~{N}-[(2~{R})-2-(4-nitrophenyl)-2-oxidanyl-ethyl]-1,3-benzodioxole-5-carboxamide | 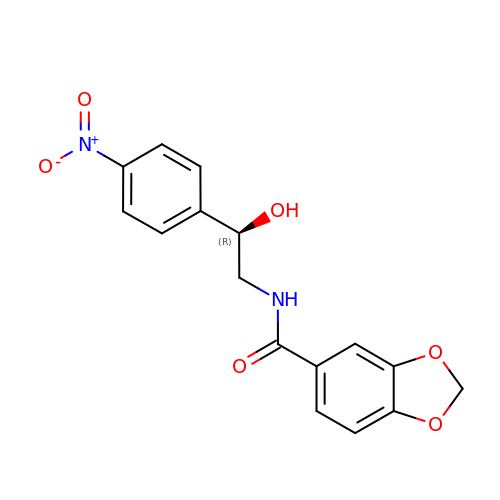C16 H14 N2 O6 | GNQZCOZNCNCXMO-ZDUSSCGKSA-N> SNAASDLYPLPAPIIDVFPDEGLAKDMAKNLNKDSVNDVIDQDDLDALTGLGFETETITNDSMQLLERAMFNNVNIVSVMEFGEDLTEFPDISTIPHLNTLFFNTPPEGVTRNLSLPDYQNY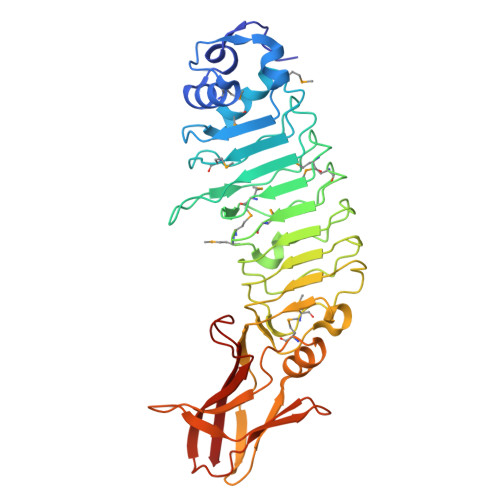PEMVTITMSGSNLIGAIPDFTGMPDLSQLYMADMMITSDDVPDFHTIPKLSTLDLSHNQLTNLPDFQNLTNLAELNLSFNNLTNTMTNFTNLSNLNNLNLDYNHLNELPSNVLNSIFIENQSGTVPDQIIKQGETCTIQLPIYFQLAEINMLVNPTVLGSYSADIPVEVVTTTNADTESITLDTSELSPGVYNFNVQFNDAYPITQEGCVYDWVLTVN>[2x]MAEIPKEMLRAQT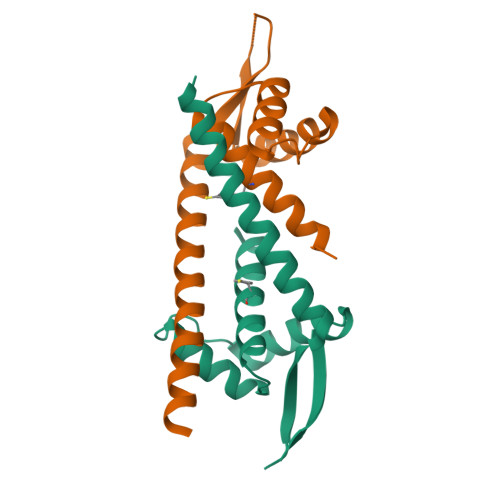NAILLNVLKQGDNYVYGIIKQVKEASNGEMELNEATLYTIFKRLEKDGIISSYWGDESQGGRRKYYRLTEIGHENMRLAFESWSRVDKIIENLEANKKSEAIKSRWSHPQFEK> GSHMASM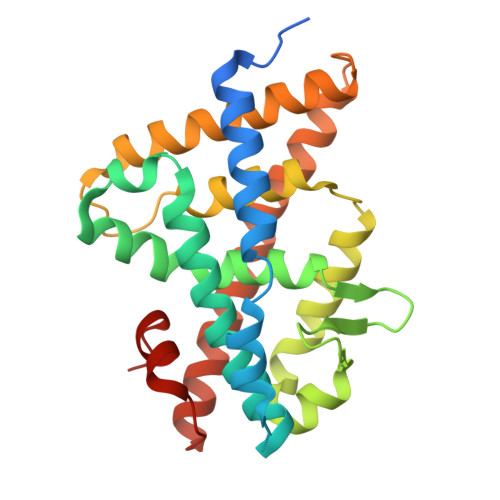TGGQQMGRDPLKNVPPLTANQKSLIARLVWYQEGYEQPSEEDLKRVTQTWQSDEDDEDSDMPFRQITEMTILTVQLIVEFAKGLPGFAKISQSDQITLLKACSSEVMMLRVARRYDAATDSVLFANNQAYTRDNYRKAGMAYVIEDLLHFCRCMYSMMMDNVHYALLTAIVIFSDRPGLEQPLLVEEIQRYYLNTLRVYILNQNSASPRCAVIFGKILGILTEIRTLGMQNSNMCISLKLKNRKLPPFLEEIWDVADVA>KFGWIKGVLVRCMLNIWGVMLFIRLSWIVGQAGIGLSVLVIMMATVVTTITGLSTSAIATNGFVRGGGAYYLISRSLGPEFGGAIGLIFAFANAVAVAMYVVGFAETVVELLKEHSILMIDEINDIRIIGAITVVILLGISVAGMEWEAKAQIVLLVILLLAIGDFVIGTFIPLESKKPKGFFGYKSEIFNENFGPDFREEETFFSVFAIFFPAATGILAGANISGDLADPQSAIPKGTLLAILITTLVYVGIAVSVGSCVVRDATGNVNDTIVTELTNCTSAACKLNFDFSSCESSPCSYGLMNNFQVMSMVSGFTPLISAGIFSATLSSALASLVSAPKIFQALCKDNIYPAFQMFAKGYGKNNEPLRGYILTFLIALGFILIAELNVIAPIISNFFLASYALINFSVFHASLAKSPGWRPAFKYYNMWISLLGAILCCIVMFVINWWAALLTYVIVLGLYIYVTYKKPDVNWGSSTQALTYLNALQHSIRLSGVEDHVKNFRPQCLVMTGAPNSRPALLHLVHDFTKNVGLMICGHVHMGPRRQAMKEMSIDQAKYQRWLIKNKMKAFYAPVHADDLREGAQYLMQAAGLGRMKPNTLVLGFKKDWLQADMRDVDMYINLFHDAFDIQYGVVVIRLKEGLDISHLQGQEELLSSQEKSPGTKDVVVSVEYSKKSDLDTSKPLSEKPITHKVEEEDGKTATQPLLKKESKGPIVPLNVADQKLLEASTQFQQKQGKNTIDVWWLFDDGGLTLLIPYLLTTKKKWKDCKIRVFIGGKIN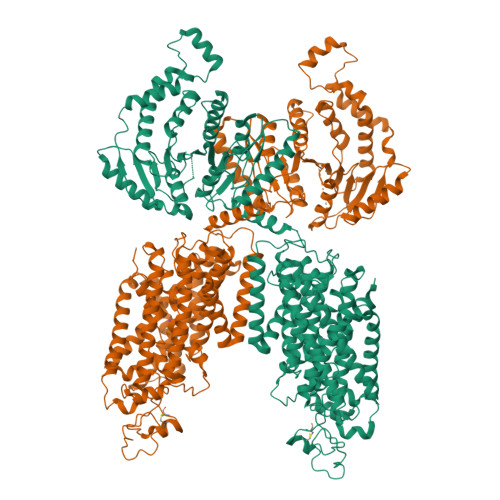RIDHDRRAMATLLSKFRIDFSDIMVLGDINTKPKKENIIAFEEIIEPYRLHEDDKEQDIADKMKEDEPWRITDNELELYKTKTYRQIRLNELLKEHSSTANIIVMSLPVARKGAVSSALYMAWLEALSKDLPPILLVRGNHQS[2x]> GAMAEEATFTANFKDTDLKSFIETVGANLNKTIIMGPGVQGKVSIRTMTPLNERQYYQLFLNLLEAQGYAVVPMYIDTNNDGYIEGDELVLKVVKSSAAKVEPLPLVGEGSDNYAGDEMVTKVVPVRNVSVRELAPILRQMIDSAGSGNVVNYDPSNVIMLTGRASVVE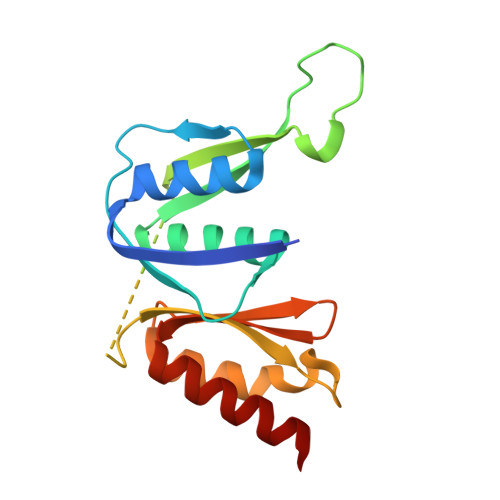RLTEVIQRVDHA>[2x]LSWKRCAGCGGKIADRFLLYAMDSYWHSRCLKCSSCQAQLGDIGTSSYTKSGMILCRNDYIRLFGNSGACSACGQSIPASELVMRAQGNVYHLKCFTCSTCRNRLVPGDRFH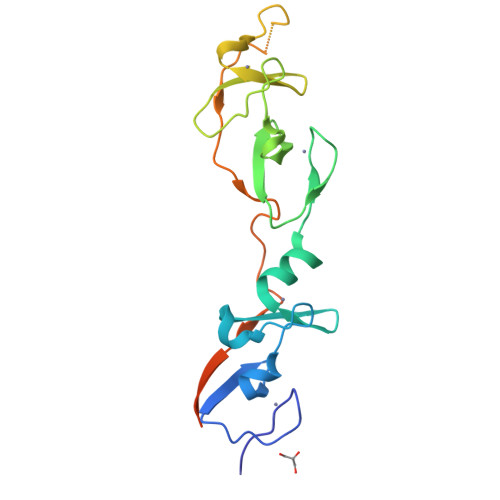YINGSLFCEHDRPTALINGHLNSGGSGGSGGSGGDVMVVGEPTLMGGEFGDEDERLITRLENTQFDAANGIDDETRESGSIEF> THDSSIRYL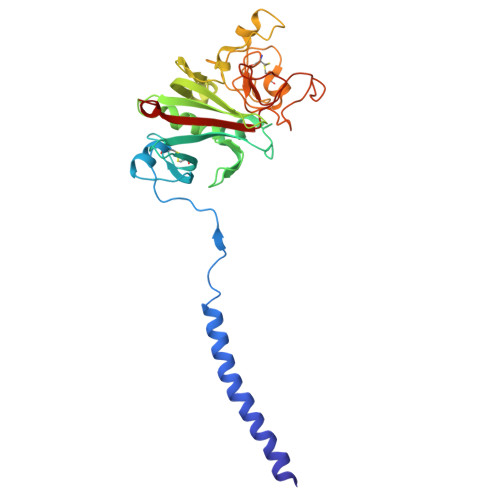QEIYNSNNQKIVNLKEKVAQLEAQCQEPCKDTVQIHDITGKDCQDIANKGAKQSGLYFIKPLKANQQFLVYCEIDGSGNGWTVFQKRLDGSVDFKKNWIQYKEGFGHLSPTGTTEFWLGNEKIHLISTQSAIPYALRVELEDWNGRTSTADYAMFKVGPEADKYRLTYAYFAGGDAGDAFDGFDFGDDPSDKFFTSHNGMQFSTWDNDNDKFEGNCAEQDGSGWWMNKCHAGHLNGVYYQGGTYSKASTPNGYANGIIWATWKTRWYSMKKTTMKIIPFNRLTI> ARILVLGLDNAGKTTILKALSEEDITTITPTQGFNIKSLSRDGFNLKIWDIGGQKSIRPYWRNYFDQTDALIYVIDSADSKRLSESEFELTELLQEEKMTGVPLLVFANKQDLVGALAADEIASTLDLTSI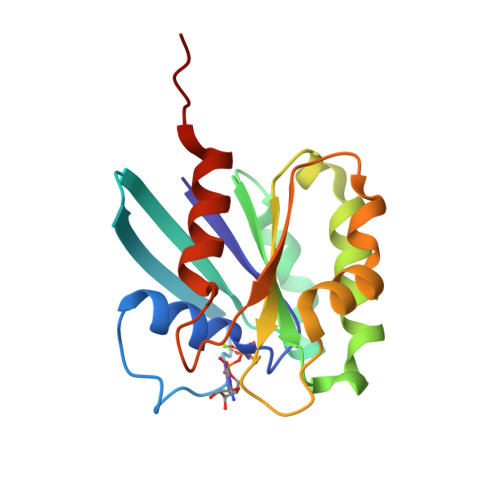RDRPWQIQACSAKQGTGLKEGMEWMMKQVKLEHHHHHH>MQLFDLSLEELKKYKPKKTARPDFSDFWKKSLEELRQVEAEPTLESYDYPVKGVKVYRLTYQSFGHSKIEGFYAVPDQTGPHPALVRFHGYNASYDGGIHDIVNWALHGYATFGMLVRGQGGSEDTSVTPGGHALGWMTKGILSKDTYYYRGVYLDAVRALEVIQSFPEVDEHRIGVIGGSQGGALAIAAAALSDIPKVVVADYPYLSNFERAVDVALEQPY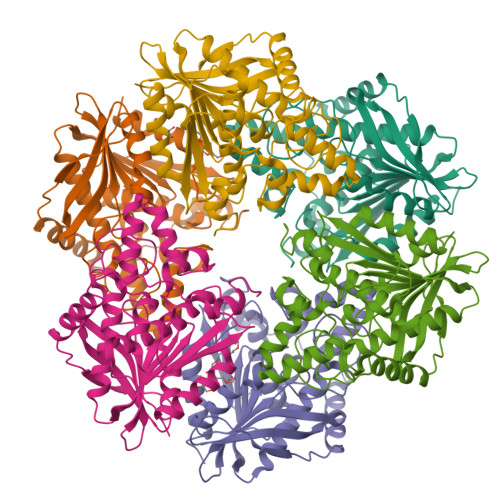LEINSYFRRNSDPKVEEKAFETLSYFDLINLAGWVKQPTLMAIGLIDKITPPSTVFAAYNHLETDKDLKVYRYFGHEFIPAFQTEKLSFLQKHLLLST[12x]CYCLOHEXYL-{4-[5-(3,4-DICHLOROPHENYL)-2-PIPERIDIN-4-YL-3-PROPYL-3H-IMIDAZOL-4-YL]-PYRIMIDIN-2-YL}AMINE | C27 H34 Cl2 N6 | 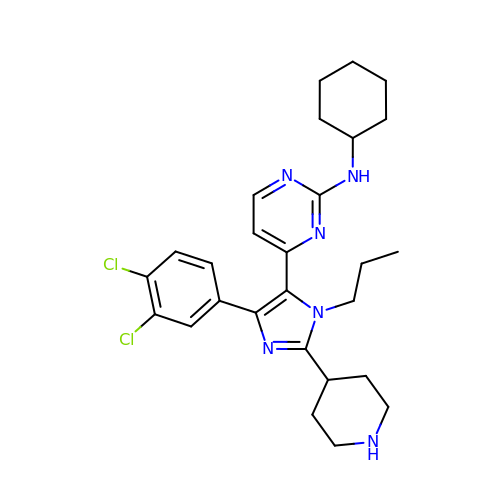UQFRSHRWRKYNDE-UHFFFAOYSA-N> UAGCUCC;> GGU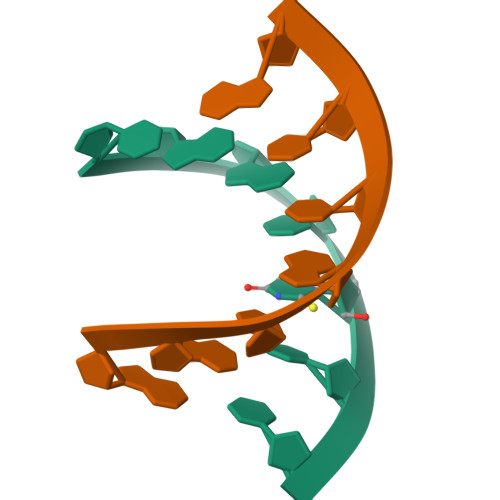GCUA>MRAEGLGGLERFCSPGKGRGLRALQPFQVGDLLFSCPAYAYVLTVNERGNHCEYCFTRKEGLSKCGRCKQAFYCNVECQKEDWPMHKLECSPMVVFGENWNPSETVRLTARILAKQKIHPERTPSEKLLAVKEFESHLDKLDNEKKDLIQSDIAALHHFYSKHLGFPDNDSLVVLFAQVNCNGFTIEDEELSHLGSAIFPDVALMNHSCCPNVIVTYKGTLAEVRAVQEIKPGEEVFTSYIDLLYPTEDRNDRLRDSYFFTCECQECTTKDKDKAKVEIRKLSDPPKAEAIRDMVRYARNVIEEFRRAKHYKSPSELLEICELSQEKMSSVFEDSNVYMLHMMYQAMGVCAYMQDAEGALQYGQKIIKPYSKHYPLYSLNVASMWLKLGRLYMGLEHKAAGEKALKKAIAIMEVAHGKDHPYISEIKQEIESH[2x]

Here, we present the discovery of a promiscuous allosteric site in SMYD2, a unique member of the protein lysine methyltransferase family characterized by the co-presence of the SET and MYND domains. SMYD2 is a critical regulator of numerous cellular processes, methylating both histone and non-histone proteins to control chromatin remodeling, DNA damage response, cell cycle progression, cell differentiation, cell survival, and inflammation. We have determined four crystal structures of SMYD2, including a wild-type protein structure in complex with a PARP1 peptide, a wild-type protein structure in complex with an ethylene glycol polymer (PEG), and two structures of SMYD2 mutants. In all structures, SMYD2 maintains a bilobal fold, with the N- and C-lobes displaying a similar orientation and a similar degree of opening.

L351A/W356A is a secondary-binding-site mutation that targets both subsites M and L, while F184A targets the target lysine access channel at the active site. In the L351A/W356A mutant structure, neither the secondary binding site nor the substrate binding site contains a peptide, although the PARP1 peptide was included during crystallization. This result suggests two possibilities: one is that this mutation disrupts binding at both sites, and the other is that the binding of the peptide to the substrate binding site depends on another peptide binding to the secondary binding site. Comparing the wild-type and mutant structures reveals that the mutation disrupts the integrity of the secondary binding site, making it less defined, explaining the loss of binding there. The most notable one is a slight movement of helices L, M, N, and O relative to helix P. This movement is likely allowed due to the extra space created by the mutation. Consistently, the substrate binding site, located about 8 Å from the mutation site, remains largely unaffected by the mutation. Strikingly, the L351A/W356A mutation completely abolished peptide binding, as evidenced by the absence of ITC heat changes. This indicates that this mutation disrupts both binding sites, consistent with the L351A/W356A mutant structure, where neither site binds to a peptide or PEG. Strikingly, the L351A/W356A mutation shifts the kinetic profile from sigmoidal to classic Michaelis-Menten kinetics, exhibiting single-site hyperbolic kinetic behavior. The L351A/W356A mutation results in a more than 10-fold increase in Vmax, while KM, which reflects apparent substrate binding affinity, shows a 4-fold increase.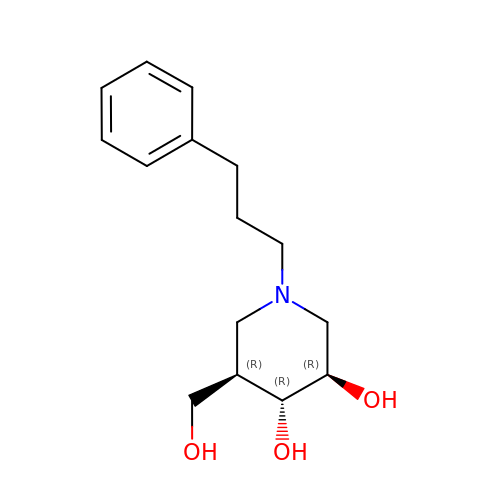(3R,4R,5R)-5-(HYDROXYMETHYL)-1-(3-PHENYLPROPYL)PIPERIDINE-3,4-DIOL | C15 H23 N O3 | NKARZGURZMIRMA-RBSFLKMASA-N>[4x]MLPGTFFEVLKNEGVVAIATQGEDGPHLVNTWNSYLKVLDGNRIVVPVGGMHKTEAN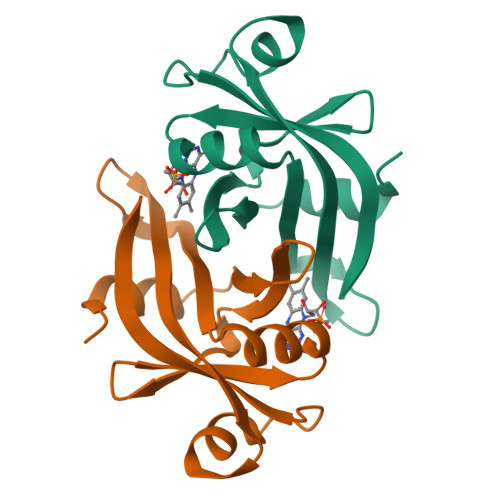VARDERVLMTLGSRKVAGRNGPGTGFLIRGSAAFRTDGPEFEAIARFKWARAALVITVVSAEQTE>MVLYFIGLGLYDERDITVKGLEIAKKCDYVFAEFYTSLMAGTTLGRIQKLIGKEIRVLSREDVELNFENIVLPLAKENDVAFLTPGDPLVATTHAELRIRAKRAGVESYVIHAPSIYSAVGITGLHIYKFGKSATVAYPEGNWFPTSYYDVIKENAERGLHTLLFLDIKARKRMYMTANEAMELLLKVEDMKKGGVFTDDTLVVVLARAGSLNPTIRAGYVKDLIREDFGDPPHILIVPGKLH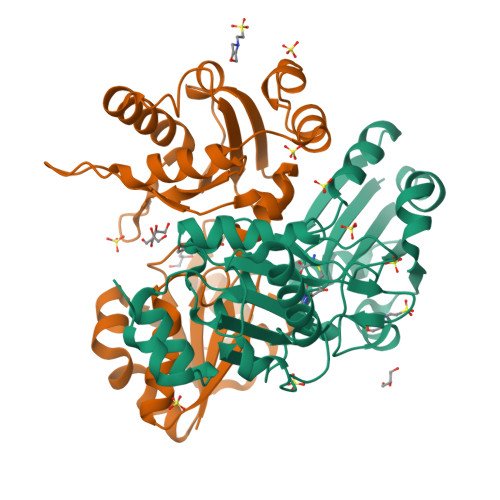IVEAEYLVEIAGAPREILRVNV[2x]> ESGKASSSLGLQDFDLLRVIGRGSYAKVLLVRLKKTDRIYAMKVVKKELVNDDEDIDWVQTEKHVFEQASNHPFLVGLHSCFQTESRLFFVIEYVNGGDLMFHMQRQRKLPEEHARFYSAEISLALNYLHERGIIYRDLKLDNVLLDSEGHIKLTDYGMCKEGLRPGDTTSTFCGTPNYIAPEILRGEDYGFSVDWWALGVLMFEMMAGRSPFDIVGSSDNPDQNTEDYLFQVILEKQIRIPRSLSVKAASVLKSFLNKDPKERLGCHPQTGFADIQGHPFFRNVDWDMMEQKQVVPPF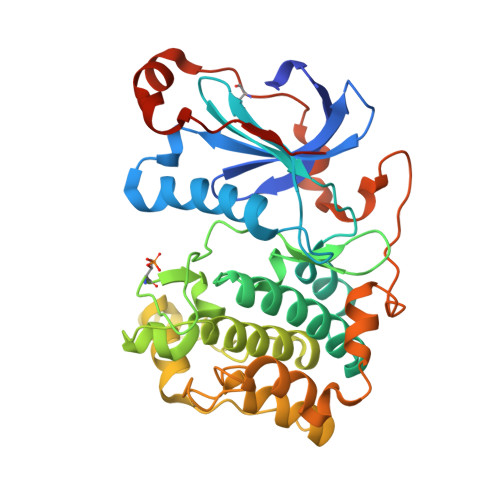KPNISGEFGLDNFDSQFTNEPVQLTPDDDDIVRKIDQSEFEGFEYINPLLMSAEECV7-(pyridin-3-ylmethyl)quinolin-8-ol 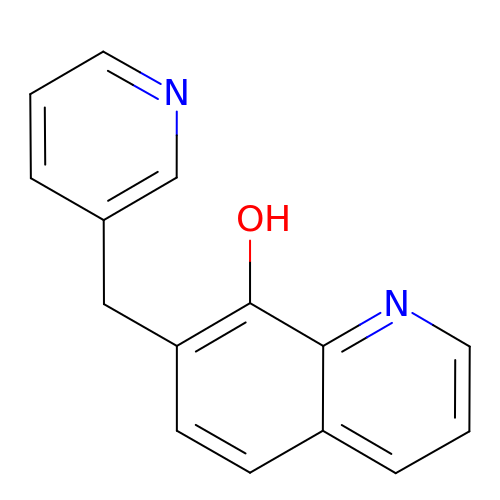| C15 H12 N2 O | DNRIDZXSDROVMC-UHFFFAOYSA-N> MACLASVALGSLHVEESLEMRFAAFKKKYGKVYKDAKEEAFRFRAFEENMEQAKIQAAANPYATFGVTPFSDMTREEFRARYRNGASYFAAAQKRLRKTVNVTTGRAPAAVDWREKGAVTPVKDQGQCGSAWAFSTIGNIEGQWQVAGNPLVSLSEQMLVSCDTIDFGCGGGLMDNAFNWIVNSNGGNVFTEASYPYVSGNGEQPQCQMNGHEIGAAITDHVDLPQDEDAIAAYLAENGPLAIAVDATSFMDYNGGILTSCTSEQLDHGVLLVGYNDASNPPYWIIKNSWSNMWGEDGYIRI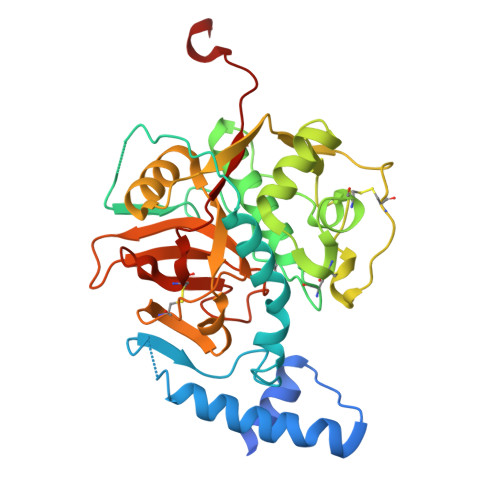EKGTNQCLMNQAVSSAVVGGPENLYFQ>QSTEASPKRHHHHHHHHHHSDENLYFQGTPFPWNKIRLPEYVIPVHYDLLIHANLTTLTFWGTTKVEITASQPTSTIILHSHHLQISRATLRKGAGERLSEEPLQVLEHPRQEQIALLAPEPLLVGLPYTVVIHYAGNLSETFHGFYKSTYRTKEGELRILASTQFEPTAARMAFPCFDEPAFKASFSIKIRREPRHLAISNMPLVKSVTVAEGLIEDHFDVTVKMSTYLVAFIISDFESVSKITKSGVKVSVYAVPDKINQADYALDAAVTLLEFYEDYFSIPYPLPKQDLAAIPDFQSGAMENWGLTTYRESALLFDAEKSSASSKLGITMTVAHELAHQWFGNLVTMEWWNDLWLNEGFAKFMEFVSVSVTHPELKVGDYFFGKCFDAMEVDALNSSHPVSTPVENPAQIREMFDDVSYDKGACILNMLREYLSADAFKSGIVQYLQKHSYKNTKNEDLWDSMASIGGGGVDVKTMMNTWTLQKGFPLITITVRGRNVHMKQEHYMKGSDGAPDTGYLWHVPLTFITSKSDMVHRFLLKTKTDVLILPEEVEWIKFNVGMNGYYIVHYEDDGWDSLTGLLKGTHTAVSSNDRASLINNAFQLVSIGKLSIEKALDLSLYLKHETEIMPVFQGLNELIPMYKLMEKRDMNEVETQFKAFLIRLLRDLIDKQTWTDEGSVSERMLRSQLLLLACVHNYQPCVQRAEGYFRKWKESNGNLSLPVDVTLAVFAVGAQSTEGWDFLYSKYQFSLSSTEKSQIEFALCRTQNKEKLQWLLDESFKGDKIKTQEFPQILTLIGRNPV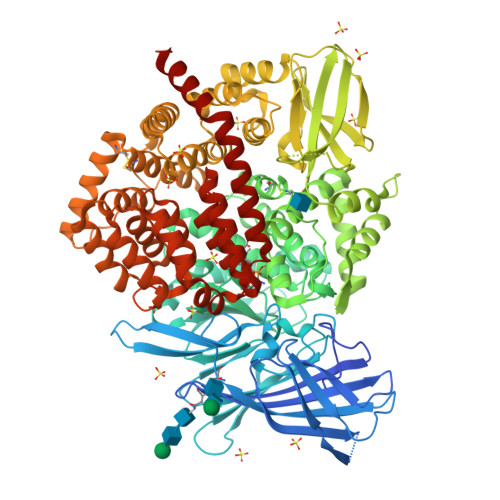GYPLAWQFLRKNWNKLVQKFELGSSSIAHMVMGTTNQFSTRTRLEEVKGFFSSLKENGSQLRCVQQTIETIEENIGWMDKNFDKIRVWLQSEKLER[22x]>SILATPILIPENQRPPFPRSVGKVIRSEGTEGAKFRLSGKGVDQDPKGIFRINEISGDVSVTRPLDREAIANYQLEVEVTDLSGKIIDGPVRLDISVIDQNDNRPMFKEGPYVGHVMEGSPTGTTVMRMTAFDADDPSTDNALLRYNILKQTPTKPSPNMFYIDPEKGDIVTVVSPVL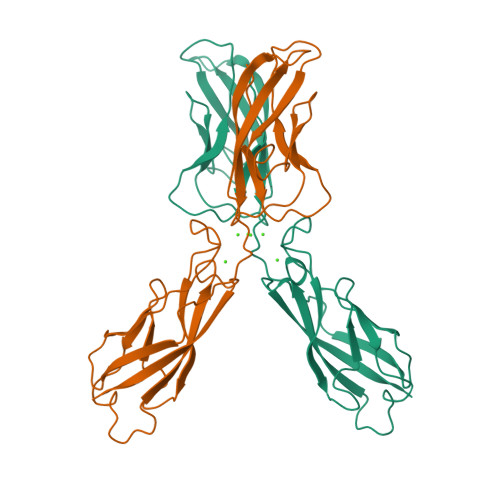LDRETMETPKYELVIEAKDMGGHDVGLTGTATATILIDD[2x]>SNAMTGPKQQPLPPDVEGREDAIEVLRAFVLDGGLSIAFMRAFEDPEMWGLLLVDIARHAARSYARESEYTEDEALERIVEMF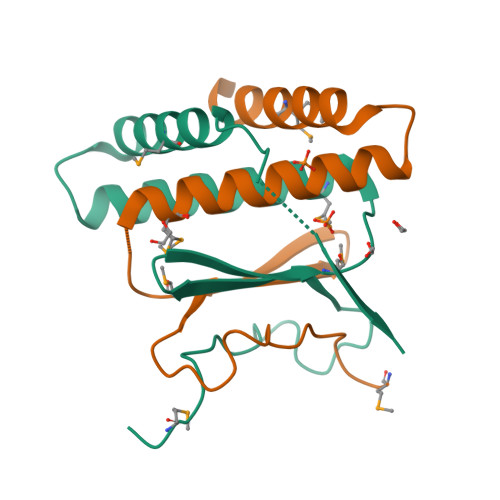EAELSRPTDTGATTERTQ[4x]O-glycosylation of the protein CST1 by the mucin-type O-glycosyltransferase T. gondii (Txg) GalNAc-T3 influences cyst wall rigidity and stability. The strict glycopeptide-preferring enzyme TxgGalNAc-T3 then adds GalNAc to acceptor Thr one position N-terminal to existing Thr-O-GalNAcs and is predicted to sequentially O-glycosylate Thr rich repeats within the mucin domain of CST1. The structures reveal a unique GalNAc binding pocket that dictates the substrate preference of TxgGalNAc-T3, which is coupled to a 2nd metal binding site that is strictly conserved among apicomplexan homologs.

To examine the role of Mn2+N in catalysis, we first verified its presence by solving the x-ray crystal structure of apo TxgGalNAc-T3 in the absence of Mn2+ to 2.9 Å resolution and did not observe density for Mn2+N. We initially hypothesized that Mn2+N was aligning the sidechains for GalNAc binding. However, a comparison of the substrate-bound structure and apo structure shows that the Mn2+N binding residues adopt similar conformations in both structures, indicating that Mn2+N uses an alternate mechanism to influence activity. Loop II is disordered in the apo structure and becomes more ordered upon peptide substrate binding.

> GARDVQEGVSSFEESGGAQLPPRVHALEVLEGAGPGRLHGRLGIKPDGQPGYTRAPSPPTDLSMPQALARGGGFNLYLSDHLELDRTAPDARHASCRQLHYDLSTLPKASVIIVFYNEPFSTLMRSVHSVLNGTPPQILEELILVDDGSTLPYIREDGNQQLVEYLKLLPAKVRLIRNEVRKGIVGARMKGIRASRAPIFAILDSHIEVSPQWLEPLLLRIKEDSRRVVMPQIDGIDAETFKHIAGGIGCKLGFLWKLMEHSYEGHQTARLPPEERQPSPTDFQTSPAMAGGLFAANKAFFFDVGAYDEDFQFWGTENLELSFRLWQCGGVLECAPCSRVYHIFRKGGSGYSSPGDSITINKMRTMLWMDEYADLAWRVIGKPRVNYRPESLEKRREWRKRKGCKSFRWFMENVFPEGDVVTLDDVPYLGPLRNDKIGMCLDNMGWASPGHAVGLEYCHGGDTQTFMFFRKVGHVMPVNDDEACLQPSGRLDWCRGTAQFWWDFTSSGQLMFRETKQCLSAFGRKLRMVECDDTDPYQIWSWTAYNPPDTFTFPSVSRSIRSG>[2x]VPRGSSKRPIRIIQWGCG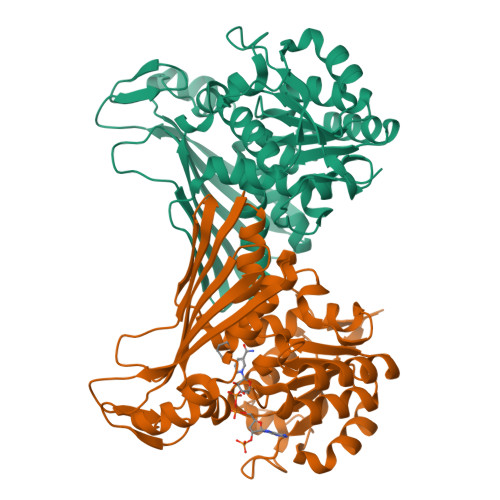LMGQTLIRTLREKGAELVGAIDHNAARRDRDAGEVAGLGQSLGVRIHPPDQADAVFREARADVCILCTRSIMSELAGALRVAARHGVNAITIGEEAFYPWTTSQALTEELDQLARANDCTLTGSGFQDVFWGNLITVLAGATHRIDRIVGLTQYNADDYGSALAQKHGVGLDPETFAARIGASNSPSYVWNSNEWLCAQLGWRVRDIRQQLLPTTHTGTLRSASLGREVPAGHATGMKAVVVTETHEGPVIETHCVGKLYAPGEVDLNEWTLRGEPDTTVTIRQPATPALTCATVLNRLPQLLAAPPGFVTTDRFTPATYVSRLETEA> SAFAPDFKELDE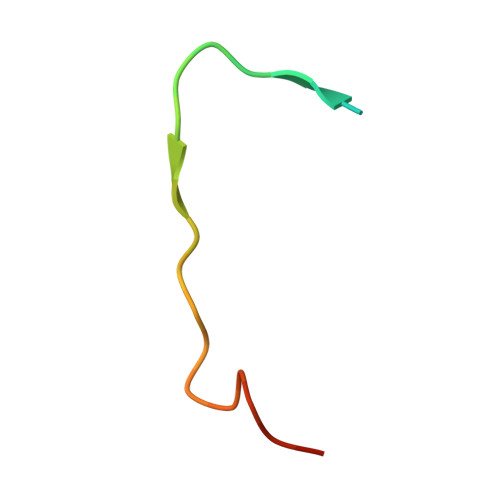NVEYEERESEFDIED[(2R,3S,4R,5R)-5-(6-amino-9H-purin-9-yl)-3,4-dihydroxytetrahydrofuran-2-yl]methyl (2R,3S,4S)-5-(8-formyl-7-methyl-2,4-dioxo-3,4-dihydrobenzo[g]pteridin-10(2H)-yl)-2,3,4-trihydroxypentyl dihydrogen diphosphate | C27 H31 N9 O16 P2 | 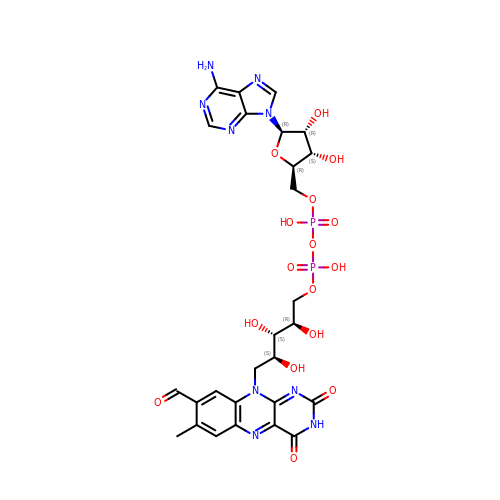WPPWMPSQWPJDHE-UYBVJOGSSA-N> MDILLVCLRF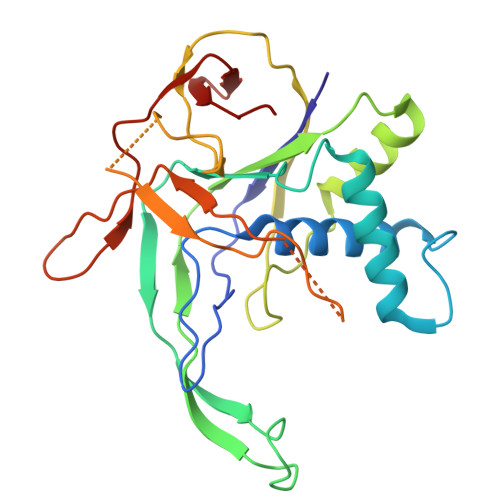PFFSVAKRSYQVRTSFLLPPPSALKGALAKGLILLKPEKYASSSLDEAALKAIKEIESKLVDIKAVSVAPLSPLIRNAFLLKRLRNLESGSNAEKSDAMRREYTFTRELLVAYIFKNLTQEEKNLYLKAAMLIDVIGDTESLATPVWASFVKPEDKKAPLAFSAPYTEIYSLLSSKIQAKGKIRMYIEKMRVSPEYSKTKGPQEEIFYLPIEERRYKRIVYYARIYPPEVEKALTVDGEVLGIWIP LDH and MDH are homologous, 2-ketoacid oxidoreductases that share both a protein fold (Rossmann et al., 1975) and a common catalytic mechanism (Birktoft and Banaszak, 1983; Clarke et al., 1986; Hart et al., 1987a, 1987b; Clarke et al., 1988; Waldman et al., 1988). Both enzymes are found in central metabolism: MDH catalyzes the interconversion of oxaloacetate and malate in the citric acid cycle, and LDH converts pyruvate to lactate in the final step of anaerobic glycolysis. A key event in the early evolution of the Apicomplexa was the acquisition of a malate dehydrogenase (MDH) via lateral gene transfer from α-proteobacteria. Following a gene duplication event roughly 700–900 Mya, one copy of this MDH evolved a novel substrate specificity to become a highly specific lactate dehydrogenase (LDH) that is now essential to the life cycle of many modern apicomplexans.

In order to understand the structural changes during evolution that shifted the enzymatic substrate specificity of the apicomplexan dehydrogenases, we determined the high-resolution crystal structures of three ancestral proteins bracketing the key duplication event: AncMDH2, AncLDH*, and AncMDH2-INS. Each protein was crystallized with multiple substrates or ligands (lactate, malate, and oxamate inhibitor) and with NADH (resolution ranging from 1.35 Å to 2.05 Å). Unfortunately, in all crystals with malate, the malate spontaneously converted to pyruvate and/or lactate via redox reactions and decarboxylation. The alternative AncMDH2 (AncMDH2*) differs from AncMDH2 by 27 residues; the alternative AncLDH (AncLDH*) differs from AncLDH by 19 residues. AncMDH2* is a strict MDH, and AncLDH* is a strict LDH. The ancestral AncLDH* and modern apicomplexan LDH structures are likewise highly similar (Winter et al., 2003; Cameron et al., 2004; Kavanagh et al., 2004) (RMSD ∼0.8 Å for the loop-closed states), while sharing only 63–71% sequence identity. The first shell active site residues are identical in the AncLDH* and modern Toxoplasma LDHs, comprising the same residues as the apicomplexan MDH active site with the sole exception of position 102, which is replaced by Trp107f in the LDHs. In both the ancestral and modern LDH structures, Trp107f and Arg109 are the only residues from the specificity loop that interact with the substrate. As in the modern LDH structures, ancestral Lys102 does not interact with the substrate but points away from the active site into solution. In contrast, Trp107f is buried within the active site, with the edge of the indole ring interacting with the pyruvate C3 methyl, which is the very chemical moiety that distinguishes pyruvate from oxaloacetate.

>[4x]MTGTMTKRKKISLIGSGMIGGTMAYLCAQKELGDVVLFDVVKNMPQGKALDLSHSSSIADTNVKVTGTNSYEDIKGSDVVIITAGLTKAPGKSDKEWSRDDLLPFNAKIMREVGENIKKYCPNAFVIVITNPLDVMVKVLHEHSGLPKNKVCGMAGVLDSSRFRHFIAEKLNVSPRDVQAMVIGAHGDKMVPLTRYVTVNGIPLQEFIKKGRITQEEIDEIVERTKNAGGEIVNLLGQGSAYFAPAASAIEMAEAYLKDKKRVLVCSCYLEGQYGHKDMFVGVPAVIGGNGVEKVIELELTPEEKELFDKSVEEVRKLQKAIKALGLEHHHHHH Here, we obtained the true atomic resolution structure of their methane-capturing system (Methyl-Coenzyme M Reductase, MCR), circumventing the isolation barrier by exploiting microbial enrichments of freshwater nitrate-reducing ANME-2d grown in bioreactors, and marine ANME-2c in syntrophy with bacterial partners. Methane capture, the first reaction in AOM, has been proposed to be carried out by the Methyl-Coenzyme M Reductase (MCR). In the proposed mechanism, the heterodisulfide, made of Coenzyme M (HS-CoM) and Coenzyme B (CoB-SH), would react with methane to generate methyl-S-CoM and free CoB-SH through a radical mechanism catalysed by the Ni-containing tetrapyrrole cofactor F43019,20. Despite their physiological differences, these ANMEs have extremely conserved MCR structures, similar to homologs from methanogenic Methanosarcinales, rather than the phylogenetically distant MCR of ANME-1 isolated from Black Sea mats.

Here, the original sample used to initiate the enrichment was collected from the Amon Mud Volcano in the Mediterranean Sea at a depth of 1120 m and a temperature of 14 °C. The microbial enrichment, grown at 20 °C in batch serum bottles since 2003, mainly gathered ANME-2c (with a relative abundance of 32%) along with microbial partners based on 16S rRNA gene sequencing7. The dataset obtained for the ANME-2c enrichment was also of sufficiently high quality to unequivocally determine the sequence from the electron density map at a resolution of 1.34 Å. The derived sequence perfectly matched the one of ANME-2c MCR from the metagenomic data. MCRs from ANME-2c and ANME-2dO contain reduced coenzymes trapped in the active site (i.e. CoM-SH and CoB-SH). ANME-2c MCR includes the conserved N1-methylhistidine and thioglycine, the common 5(S)-methylarginine, 2(S)-methylglutamine, and the rarer S-methylcysteine, didehydroaspartate, and 6-hydroxytryptophan. The dimeric interface is exclusively formed by the interaction of the α-subunits, mainly via the C-terminal extension. The dimeric state does not disturb the access to the active site. Due to the low quantities of MCR obtained at the end of the purification and the slow growth of the consortium, we were unable to test whether this dimeric arrangement reflects a crystallisation artefact or a stable entity in solution. Despite the different environmental niches, the marine ANME-2c and freshwater ANME-2d MCRs have high amino acid sequence identities of 63.6%, 61.5%, and 71.4% for α, β, and γ subunit, respectively.

>[8x]MAYKYPSEKLFVEALKSKFAGLDLSDQKVKYVRAGYLQNARKREFQAAGERVAEQRGMQQYDVNVHLGGMTLGQRQLVPYKLSTRPDIVEGDDLHYVNNPAMQQMWDDMKRTIIVGMDLAHETLEKRLGKEVTPESIAGYMEAVNHTMPGAAIVQEHMVETHPGLVDDCYVKMFTGDDELADEIDSQYVININDLFDKEGQNEKLKAAIGKTTWQAVHIPTIVVRCCDGGNTSRWSAMQIGMSFIAAYNMCAGEAAVADLAFAAKHAAAVQMAEMLPARRARSPNEPGGLSFGYCADMVQTLRVKPEDPVWYTLEVVACGTMLYDQIWLGSYMSGGVGFTQYATAAYTNDVLDDFTYYGYDYALNKYGDDGTAPNDLATATDLATEVTLNGMECYEDYPTLLEDHFGGSQRAGILAAASACTTGIATGNSQVALSAWYMSMYVHKEGWGRLGFFGYDLQDQCGATNVCSYQGDEGCCLELRGANYPNYAMNVGHQGEYAGFTGSAHAGAHDAYCCNPLIKVCFADPSLVFDFSYIRKEYAKGAMRTFRPAGERSLVIPAGV;>MADTIDLYDDRGKKLKGDVDLQAVSPLKNSAILSMVNTVKRTVAVNLAGIEKACKNASYGGQSRNIPGREVDIDPTAKADKIAARVKELIQVEKGDDTEVTVLGGGKFLRVAAPTRRIEAGAEYVAGMTCTAAALTEALREEYNLGLYDTPYVKNAVWGTYPQTMDMKGGNVLSVLSIPQNDEGLGFALRNIMANHLAMLSQRNAMNCAAISSILEHCGVFEMGQAIGLFERYQLLALAYQGLNANNMVYEMTKNNGKTGTIGTVVQETVGRALDDGVISVDKTMPSGYKVYKANDVCMWNAYCAAGTMAATMVNCGALRGAQAVSSTLLYFNDMIEKETSLPGCDWGRVEGTAVGFSFFSHSIYGGGGPGVFNGNHVVTRHSTGMAIPCVAVAVALDAGTQMFSPESTSAIVLDTFQDVPIMMNPLKEVAAAV[8x];>MAYTPQYYPGSSHVAVNRRKHMSGDVEKLRTVSDDDLVAALGHRAPGADYPSTHPPLAEMGEPDCPVRQMVEPTPGAAAGDRVRYSQFTDSMYSAPSIPYFRSYYAAINFRGVDPGTLSGRQIVEARERDMEAQCKAAIESEMTCPALAGLRGCTVHGHSLRLAEDGMMFDMLQRTHIEGGNVIEDKDQVGVPIDRKVNLGKPMSDAEAKKRTTIYRTDGVKYRDEEEVLDHVHLVHHRRTMYGYRPETAAETAPGVGPVTYHTV[8x]> MAD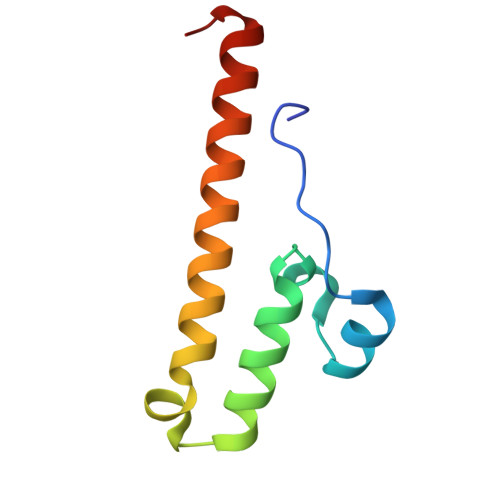RFPPPKMVATQEEMDNADIPYKYRDYCAHLIIDFKECRYGHPLTWRINCAHELHHYNKCSYIEFKRRVAIAIEEKKRRGLMV>MEALVLVGHGSRLPYSKELLVKLAEKVKERNLFPIVEIGLMEFSEPTIPQAVKKAIEQGAKRIIVVPVFLAHGIHTTRDIPRLLGLIEDNHEHHHEHSHH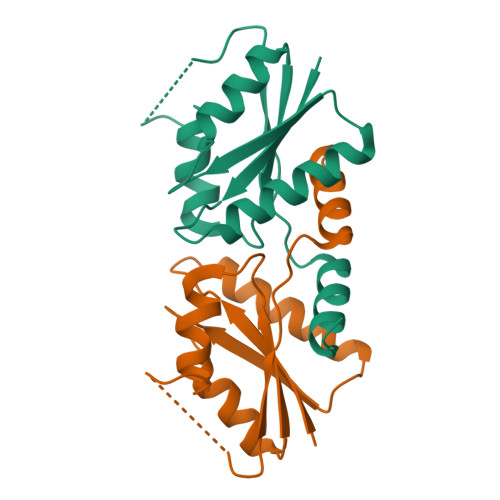HHHHHHHEHEKLEIPEDVEIIYREPIGADDRIVDIIIDRAFGR[2x]(2S)-2-azanyl-4-[[(2R)-3-(1H-imidazol-4-yl)-1-oxidanyl-1-oxidanylidene-propan-2-yl]amino]butanoic 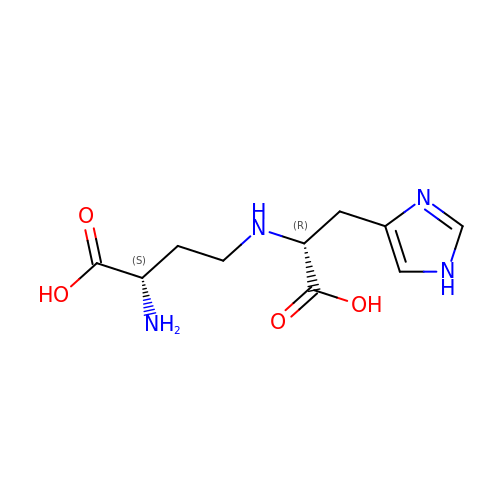acid | C10 H16 N4 O4 | PQUPEWJRDBYFHU-JGVFFNPUSA-N> KSLRV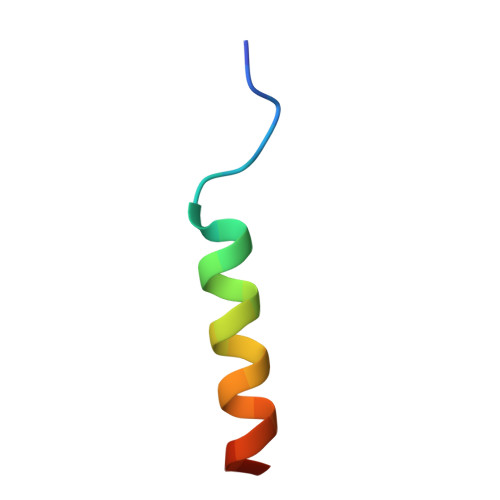SSLNKDRRLLLREFYNLEN> EDVVWRWSCDNGKCVKLKNDPRSSEPALSLEACKMFCNEYGLLWPRPTGEADLGNFLSKINLNSIEVKILKKGATDDLMEAAAKRFKEQVSLAIPRGSTPKLTGKAVDVYLVNENPNEKAFSLEMDESYGLRVSPSGADRVNATITANSFFGMRHGLETLSQLFVFDDIRDHLLMVRDVNISDKPVYPYRGILLDTARNYYSIESIKRTIEAMAAVKLNTNHWHITDSQSFPFVTTKRPNLYKFGALSPQKVYTKAAIREVVRFGLERGVRVLPEFDAPAHVGEGWQDTDLTVCFKAEPWKSYCVAPPCGQLNPTKDELYQYLEDIYSDMAEVFDTTDIFHMGGDEVSEACWNSSDSIQNFMMQNRWDLDKESFLKLWNYFQQKAQDKAYKAFGKKLPLILWTSTLTNYKHIDDYLNKDDYIIQVWTTGVDPQIKGLLEKGYRLIMSNYDALYFDCGYGAWVGAGNNWCSPY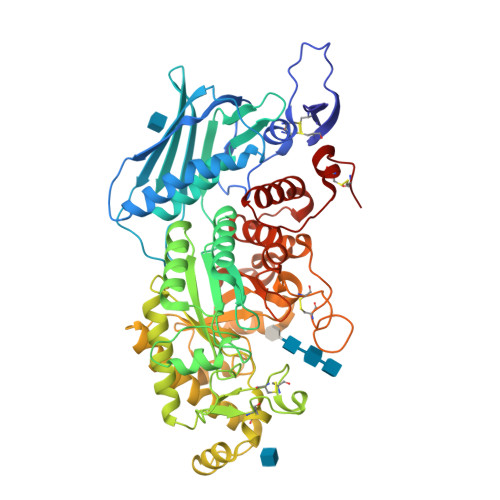IGWQKVYDNSPAVIALEHRDQVLGGEAALWSEQSDTSTLDGRLWPRAAALAERLWAEPATSWQDAEYRMLHIRERFVRMGIQAESLQPEWCYQNEGYCYS> GGUCAAGAUAGUAAGGGUCCACGGUGGAUGCCCUGGCGCUGGAGCCGAUGAAGGACGCGAUUACCUGCGAAAAGCCCCGACGAGCUGGAGAUACGCUUUGACUCGGGGAUGUCCGAAUGGGGAAACCCACCUCGUAAGAGGUAUCCGCAAGGAUGGGAACUCAGGGAACUGAAACAUCUCAGUACCUGAAGGAGAAGAAAGAGAAUUCGAUUCCGUUAGUAGCGGCGAGCGAACCCGGAUCAGCCCAAACCGAAACGCUUGCGUUUCGGGGUUGUAGGACCAGUUUUUAAGAUUCAACCCCUCAAGCCGAAGUGGCUGGAAAGCUACACCUCAGAAGGUGAGAGUCCUGUAGGCGAACGAGCGGUUGACUGUACUGGCACCUGAGUAGGUCGUUGUUCGUGAAACGAUGACUGAAUCCGCGCGGACCACCGCGCAAGG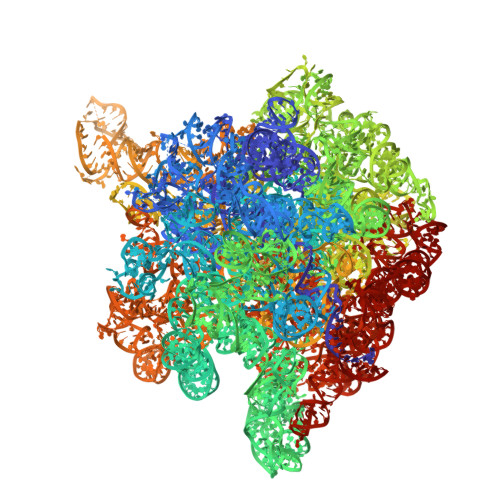CUAAAUACUCCCAGUGACCGAUAGCGCAUAGUACCGUGAGGGAAAGGUGAAAAGAACCCCGGGAGGGGAGUGAAAGAGAACCUGAAACCGUGGACUUACAAGCAGUCAUGGCACCUUAUGCGUGUUAUGGCGUGCCUAUUGAAGCAUGAGCCGGCGACUUAGACCUGACGUGCGAGCUUAAGUUGAAAAACGGAGGCGGAGCGAAAGCGAGUCCGAAUAGGGCGGCAUUAGUACGUCGGGCUAGACUCGAAACCAGGUGAGCUAAGCAUGACCAGGUUGAAACCCCCGUGACAGGGGGCGGAGGACCGAACCGGUGCCUGCUGAAACAGUCUCGGAUGAGUUGUGUUUAGGAGUGAAAAGCUAACCGAACCUGGAGAUAGCUAGUUCUCCCCGAAAUGUAUUGAGGUACAGCCUCGGAUGUUGACCAUGUCCUGUAGAGCACUCACAAGGCUAGGGGGCCUACCAGCUUACCAAACCUUAUGAAACUCCGAAGGGGCACGCGUUUAGUCCGGGAGUGAGGCUGCGAGAGCUAACUUCCGUAGCCGAGAGGGAAACAACCCAGACCAUCAGCUAAGGUCCCUAAAUGAUCGCUCAGUGGUUAAGGAUGUGUCGUCGCAUAGACAGCCAGGAGGUUGGCUUAGAAGCAGCCACCCUUCAAAGAGUGCGUAAUAGCUCACUGGUCGAGUGACGAUGCGCCGAAAAUGAUCGGGGCUCAAGUGAUCUACCGAAGCUAUGGAUUCAACUCGCGAAGCGAGUUGUCUGGUAGGGGAGCGUUCAGUCCGCGGAGAAGCCAUACCGGAAGGAGUGGUGGAGCCGACUGAAGUGCGGAUGCCGGCAUGAGUAACGAUAAAAGAAGUGAGAAUCUUCUUCGCCGUAAGGACAAGGGUUCCUGGGGAAGGGUCGUCCGCCCAGGGAAAGUCGGGACCUAAGGUGAGGCCGAACGGCGCAGCCGAUGGACAGCAGGUCAAGAUUCCUGCACCGAUCAUGUGGAGUGAUGGAGGGACGCAUUACGCUAUCCAAUGCCAAGCUAUGGCUAUGCUGGUUGGUACGCUCAAGGGCGAUCGGGUCAGAAAAUCUACCGGUCACAUGCCUCAGACGUAUCGGGAGCUUCCUCGGAAGCGAAGUUGGAAACGCGACGGUGCCAAGAAAAGCUUCUAAACGUUGAAACAUGAUUGCCCGUACCGCAAACCGACACAGGUGUCCGAGUGUCAAUGCACUAAGGCGCGCGAGAGAACCCUCGUUAAGGAACUUUGCAAUCUCACCCCGUAACUUCGGAAGAAGGGGUCCCCACGCUUCGCGUGGGGCGCAGUGAAUAGGCCCAGGCGACUGUUUACCAAAAUCACAGCACUCUGCCAACACGAACAGUGGACGUAUAGGGUGUGACGCCUGCCCGGUGCCGGAAGGUCAAGUGGAGCGGUGCAAGCUGCGAAAUGAAGCCCCGGUGAACGGCGGCCGUAACUAUAACGGUCCUAAGGUAGCGAAAUUCCUUGUCGGGUAAGUUCCGACCUGCACGAAAGGCGUAACGAUCUGGGCGCUGUCUCAACGAGGGACUCGGUGAAAUUGAAUUGGCUGUAAAGAUGCGGCCUACCCGUAGCAGGACGAAAAGACCCCGUGGAGCUUUACUAUAGUCUGGCAUUGGGAUUCGGGUUUCUCUGCGUAGGAUAGGUGGGAGCCUGCGAAACUGGCCUUUUGGGGUCGGUGGAGGCAACGGUGAAAUACCACCCUGAGAAACUUGGAUUUCUAACCUGAAAAAUCACUUUCGGGGACCGUGCUUGGCGGGUAGUUUGACUGGGGCGGUCGCCUCCCAAAAUGUAACGGAGGCGCCCAAAGGUCACCUCAAGACGGUUGGAAAUCGUCUGUAGAGCGCAAAGGUAGAAGGUGGCUUGACUGCGAGACUGACACGUCGAGCAGGGAGGAAACUCGGGCUUAGUGAACCGGUGGUACCGUGUGGAAGGGCCAUCGAUCAACGGAUAAAAGUUACCCCGGGGAUAACAGGCUGAUCUCCCCCGAGAGUCCAUAUCGGCGGGGAGGUUUGGCACCUCGAUGUCGGCUCGUCGCAUCCUGGGGCUGAAGAAGGUCCCAAGGGUUGGGCUGUUCGCCCAUUAAAGCGGCACGCGAGCUGGGUUCAGAACGUCGUGAGACAGUUCGGUCUCUAUCCGCUACGGGCGCAGGAGAAUUGAGGGGAGUUGCUCCUAGUACGAGAGGACCGGAGUGAACGGACCGCUGGUCUCCCUGCUGUCGUACCAACGGCACAUGCAGGGUAGCUAUGUCCGGAACGGAUAACCGCUGAAAGCAUCUAAGCGGGAAGCCAGCCCCAAGAUGAGUUCUCCCACUGUUUAUCAGGUAAGACUCCCGGAAGACCACCGGGUUAAGAGGCCAGGCGUGCACGCAUAGCAAUGUGUUCAGCGGACUGGUGCUCAUCAGUCGAGGUCUUGACCACUC N-[2-[2-(6-aminopurin-9-yl)ethoxy]ethyl]-5-(4-fluorophenyl)-2,3-dihydroxybenzamide 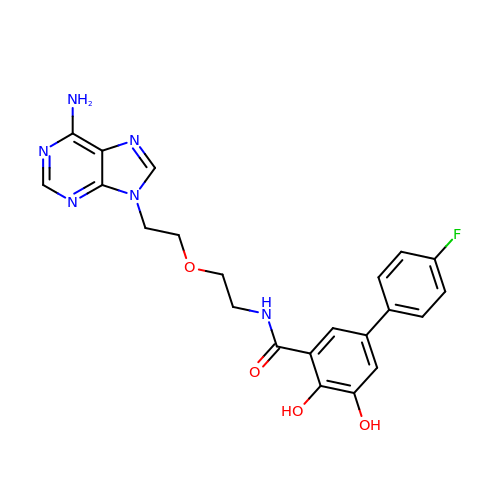| C22 H21 F N6 O4 | MBDKBZKJWMEJRT-UHFFFAOYSA-N>[4x]MTDTGTGV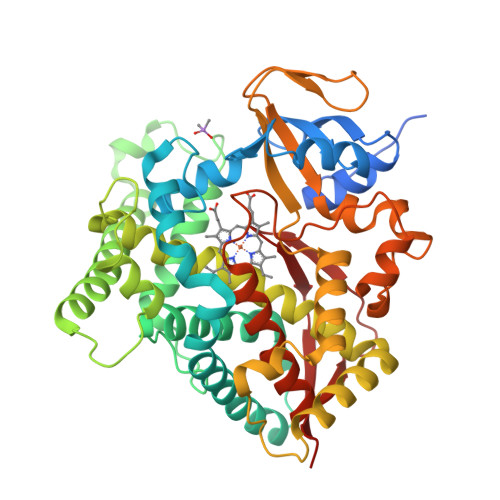HTPQPLPHPRGRLPVLRDLLSVDFATPVQGLTREGRRHDGIFEQCIGDFRVVVVDGPELIEEINNPQLWEKNVGPTLHKLRSVAGDGMFTAYNSEENWRKAHEILTPAFTKEAMSTYHQRIAATVRELIDAWNTRAQNNSWIDIPAETNRLTIEIISRAGFDYQFNNLADHSENPFITAVLRELQYANRRTDSIPFYEQFLGGRRRRLHAADKKFIRAEVDKIIDVRRINPRVGQSPDMLDIMLTAADPVTGDKLDNNNIGNQILTFLVAGSETSANAIAFALHFLATTPDVAAQARAEVDAMWPGRTFPDFQFDQIAKLRYLRLVIDEALRLWPVAPGYFRQAKQDTTIGEGRYAFKKNDWVFVNLHAAHTHRSWGPDAAEFKPERMSTENRRKLGPHIYKPFGVGERACIGRQFAQHEMVIALAAILHQFELEPRPGYELKVSETLTLKPSDLQLRLRNRV Meso-2,3-Butanediol 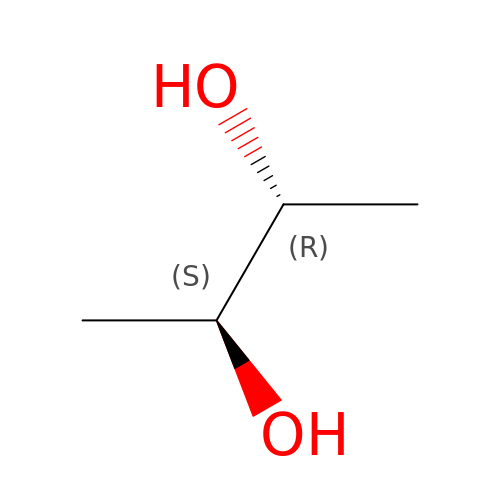| C4 H10 O2 | OWBTYPJTUOEWEK-ZXZARUISSA-N> APKAPADGLKMDKTKQPVVFNHSTMKAVKCGDCHHPVNGKEDY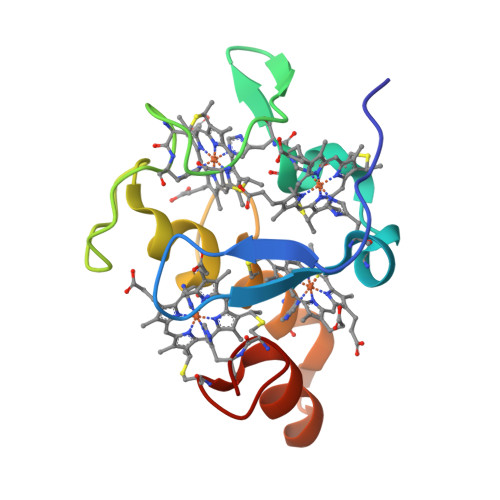QKCATAGCHDNMDKKDKSAKGYYHAMHDKGTKFKSCVGCHLETAGADAAKKKELTGCKGSKCHS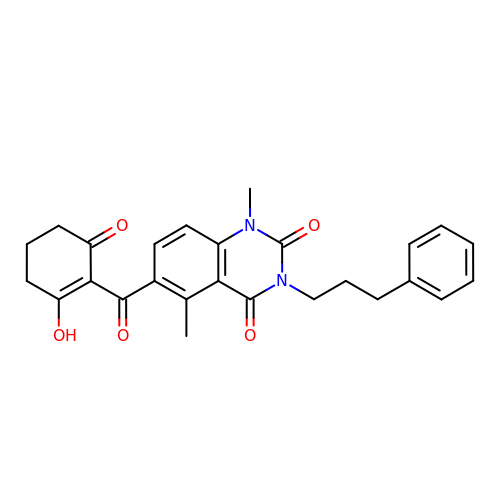1,5-dimethyl-6-(2-oxidanyl-6-oxidanylidene-cyclohexen-1-yl)carbonyl-3-(3-phenylpropyl)quinazoline-2,4-dione | C26 H26 N2 O5 | AWYNLWBZJALMMQ-UHFFFAOYSA-N>QTVARKCSLTGKWTNDLGSNMTIGAVNSRGEFTGTYITAVADNPGNITLSPLLGIQHKRASQPTFGFTVNWKFSESTTVFTGQCFIDRNGKEVLKTMWLLRSSVNDIGDDWKATRVGYNIFTRLRTQ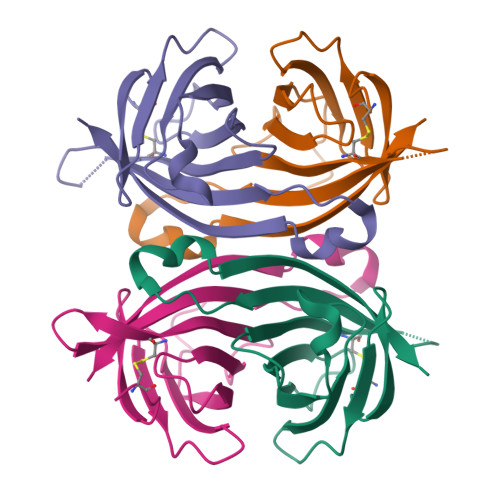KE[12x]>MGSSHHHHHHSSGLVPRGSHMAHSQSIFDIHSLTSPVLSAEEIHLIEASVEQFGAPLLLLDCDVIRQQYRALKNALPNVTLHYALKPLPHPVVVRTLLAEGASFDLATTGEVELVASEGVPADLTIHTHPIKRDADIRDALAYGCNVFVVDNLNELEKFKAYRDDVELLVRLSFRNSEAFADLSKKFGCSPEQALVIIETAKEWNIRIKGLSFHVGSQTTNPNKYVEAIHTCRHVMEQVVERGLPALSTLDIGGGFPVNYTQQVMPIDQFCAPINEALSLLPETVHVLAEPGRFICAPAVTSVASVMGQAEREGQIWYYLDDGIYGSFSGLMFDDARYPLTTI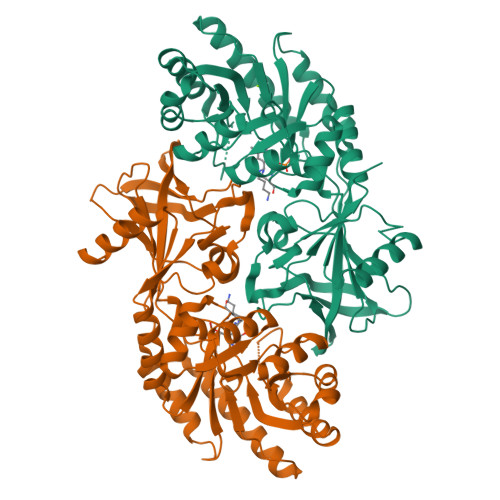KQGGELIPSVLSGPTCDSVDVIAENILLPKLNNGDLVIGRTMGAYTSATATDFNFFKRAQTIALNEFVASSERMIG[2x]>[2x]GPLGSVRDEIRSMVSDSVDEIVDGVSKTTAEVINGRKSIAQYATSLIESNPEPDNVRTIISQPLIKNTFLLVGFGLEKDGSNINNDPSWNPGPTWDPRVRPWYKDAKNAGKLVITAPYADSASGEILVSVATPVKDSATGQFLGSIFYDVSLAELAELVNEVKLFDAGYVFIVSEDGTTIAHPKKEFNGKPMSEFLGESKINVDTHQVIINGKPYAVSFSDVEGEDWYVGVVIDEEIAY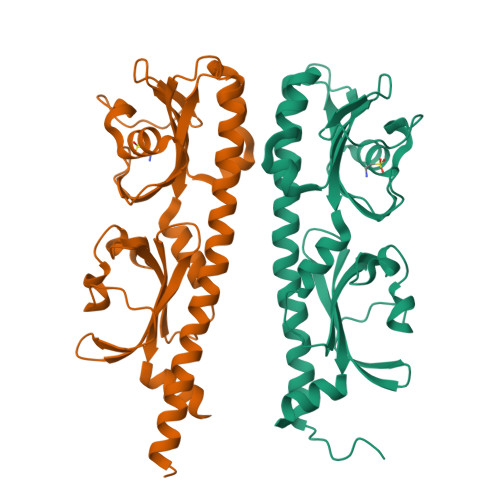AALDELRRSTLIHHHHHH> GSHMGLFNAHAVAQQRADRIATLLQSFADGQLDTAGGEAPAPGYERLYDSLRALQRQLREQRAELQQVESLEAGLAEMSRQHEAGWIDQTIPAERLEGRAARIAKGVNELVAAHIAVKMKVVSVVTAYGQGNFEPLMDRLPGKKAQIT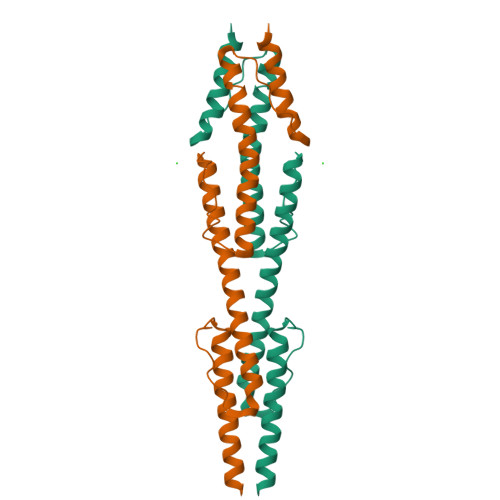EAIDGVRERLRGAAEATSAQLATAAYN>PVMKTFKEFLLSLDDSVDETEAVKRYNDYKLDFRRQQMQDFFLAHKDEEWFRSKYHPDEVGKRRQEARGALQNRLRVFLSLMETGWFDNLLLDIDKADAIVKMLDAAVIKMEGGTEND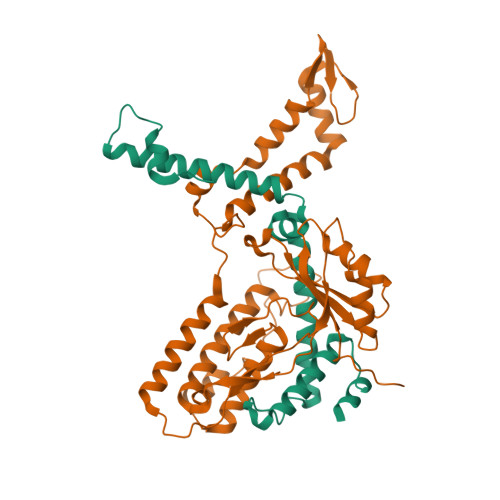LRILEQ[2x];>[2x]GLECKPRPLHKTCSLFMRNIAPNISRAEIISLCKRYPGFMRVALSEPQPERRFFRRGWVTFDRSVNIKEICWNLQNIRLRECELSPGVNRDLTRRVRNINGITQHKQIVRNDIKLAAKLIHTLDDRTQLWASEPGTPPLPTSLPSQNPILKNITDYLIEEGSGSGSERDEKLIKVLDKLLLYLRIVHSLDYYNTCEYPNEDEMPNRCGIIHVRGPMPPNRISHGEVLEWQKTFEEKLTPLLSVRESLSEEEAQKMGRKDPEQEVEKFVTSNTQELGKDKWLCPLSGKKFKGPEFVRKHIFNKHAEKIEEVKKEVAFFNNFLTDAKRPALPE hIDO1 is a heme-containing enzyme that catalyzes the first and rate-limiting step of the kynurenine pathway—the dioxygenation of Trp to N-formyl kynurenine (NFK). It negatively regulates cellular immune response via depleting Trp and promoting the accumulation of kynurenine pathway metabolites. HIDO1 is an α-helical protein, made up by a large C-terminal domain containing the Sa site and a small N-terminal domain sitting on top of it. Here we report the structures of the wild-type hIDO1 in complex with Trp, an inhibitor (epacadostat), and/or an effector (IDE), as well as comparable structures of an active site mutant, F270G.

We next crystallized the F270G-CN-Trp complex in the presence and absence of IDE, and solved their structures at a resolution of 2.69 and 3.03 Å, respectively. In the IDE complex, IDE binds to the Si site in a manner similar to that observed in the wild-type complex. Although both the IDE complex and the two Trp-bound complex of the F270G mutant exhibit impeded enzyme activity, their structures are surprisingly similar to that of the wild-type complex, except that the heme is more planar and that the protein matrix is more flexible, in particular in the regions near the JK-LoopC, the K-Helix and D-Helix, as exemplified by the ability of the R231 sidechain to adopt two conformations in the IDE complex.

>MSKEYHIDEEVGFALPNPQENLPDFYNDWMFIAKHLPDLIESGQLRERVEKLNMLSIDHLTDHKSQRLARLVLGCITMAYVWGKGHGDVRKVLPRNIAVPYCQLSKKLELPPILVYADCVLANWKKKDPNKPLTYENMDVLFSFRDGDCSKGFFLVSLLVEIAAASAIKVIPTVFKAMQMQERDTLLKALLEIASCLEKALQVFHQIHDHVNPKAFFSVLRIYLSGWKGNPQLSDGLVYEGFWEDPKEFAGGSAGQSSVGQCFDVLLGIQQTAGGGHAAQFLQDMRRYMPPAHRNFLCSLESNPSVREFVLSKGDAGLREAYDACVKALVSLRSYHLQIVTKYILIPASQQPKENKTSEDPSKLEAKGTGGTDLMNFLKTVRSTTEKSLLKEGKGELNSKLEGKPIPNPLLGLDSTRTGHHHHHH[2x]> STGSATTTPIDSLDDAYITPVQIGTPAQTLNLDFDTGSSDLWVFSSETTA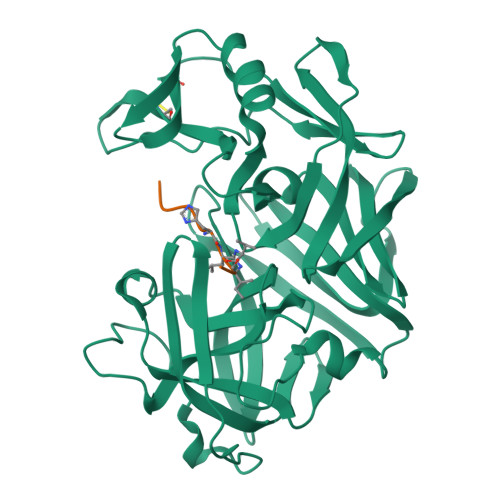SEVDGQTIYTPSKSTTAKLLSGATWSISYGDGSSSSGDVYTDTVSVGGLTVTGQAVESAKKVSSSFTEDSTIDGLLGLAFSTLNTVSPTQQKTFFDNAKASLDSPVFTADLGYHAPGTYNFGFIDTTAYTGSITYTAVSTKQGFWEWTSTGYAVGSGTFKSTSIDGIADTGTTLLYLPATVVSAYWAQVSGAKSSSSVGGYVFPCSATLPSFTFGVGSARIVIPGDYIDFGPISTGSSSCFGGIQSSAGIGINIFGDVALKAAFVVFNGATTPTLGFASK;> PHPFHXIHK> GSHMGVINKPEAEMSPQELQLHYFKMHDYDGNNLLDGLELSTA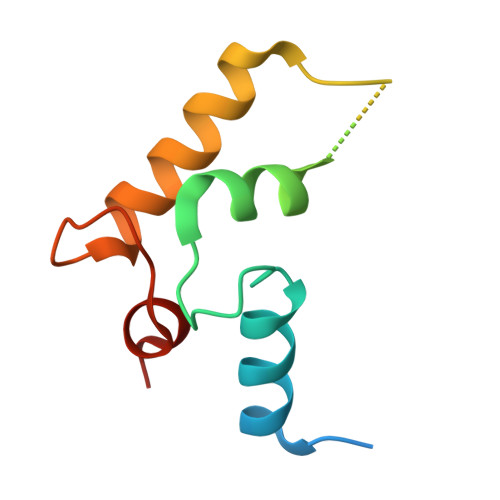ITHVHKEEGSEQAPLMSEDELINIIDGVLRDDDKNNDGYIDYAEFAKSLQ>MTTSFTDPAISMDLLRAVLQPSINEEIQTVFNKYMKFFQKAALNVRDNVGEEVDAEQLIQEACRSCLEQAKLLFSDGEKVI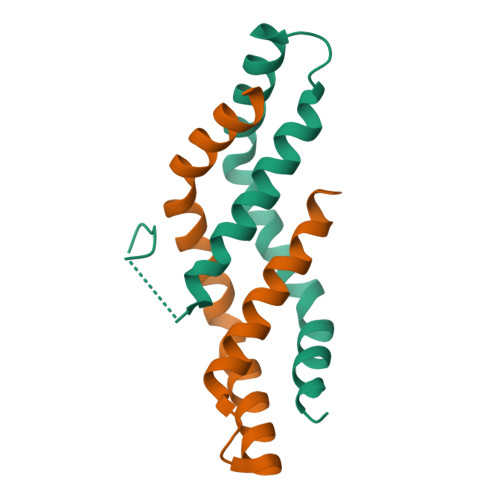PRLTHELPGIK[6x]Regnase-1 (also known as Zc3h12a and MCPIP1) is an RNase whose expression level is stimulated by lipopolysaccharides and prevents autoimmune diseases by directly controlling the stability of mRNAs of inflammatory genes such as interleukin (IL)-6, IL-1β, IL-2, and IL-12p404567. Regnase-1 accelerates target mRNA degradation via their 3′-terminal untranslated region (3′UTR), and also degrades its own mRNA8. Regnase-1 is a member of Regnase family and is composed of a PilT N-terminus like (PIN) domain followed by a CCCH-type zinc–finger (ZF) domain, which are conserved among Regnase family members. Our findings suggest that Regnase-1 cleaves its target mRNA by an NTD-activated functional PIN dimer, while the ZF increases RNA affinity in the vicinity of the PIN dimer.

X-ray crystallography was attempted for the fragment containing both the PIN and ZF domains, however, electron density was observed only for the PIN domain, consistent with a previous report on Regnase-1 derived from Homo sapiens. This suggests that the PIN and ZF domains exist independently without interacting with each other. We found that the PIN domain formed a head-to-tail oligomer that was commonly observed in all three crystal forms in spite of the different crystallization conditions. The amino acid sequences corresponding to PIN (residues 134–295) are the two non-identical residues are substituted with similar amino acids. Both the mouse and human PIN domains form head-to-tail oligomers in three distinct crystal forms. In contrast, our gel filtration data, mutational analyses, and NMR spectra all indicate that the PIN domain forms a head-to-tail dimer in solution in a manner similar to the crystal structure. The previously reported crystal structure of the Regnase-1 PIN domain derived from Homo sapiens is nearly identical to the one derived from Mus musculus in this study, with a backbone RMSD of 0.2 Å. The importance of residues W182 and R183 can readily be understood in terms of the monomeric PIN structure as they are located near to the RNase catalytic site; however, the importance of residue K184, which points away from the active site is more easily rationalized in terms of the oligomeric structure, in which the “secondary” chain’s residue K184 is positioned near the “primary” chain’s catalytic site. In contrast, R214 is important for oligomerization of the PIN domain and the “secondary” chain’s residue R214 is also positioned near the “primary” chain’s active site within the dimer interface. Within the crystal structure of the PIN dimer, the Regnase-1 specific basic regions in both the “primary” and “secondary” PINs are located around the catalytic site of the primary PIN. In the absence of target mRNA, the PIN domain forms head-to-tail oligomers at high concentration.

>GPHMDLRPVVIDGSNVAMSHGNKEVFSCRGILLAVNWFLERGHTDITVFVPSWRKEQPRPDVPITDQHILRELEKKKILVFTPSRRVGGKRVVCYDDRFIVKLAFESDGVVVSNDTYRDLQGERQEWKRFIEERLLMYSFVNDKFMPPDDPLGRHGPSLDNFLRKKPLPSEHRKQPCPYGKKCTYGIKCRFFHPERPSRPQRSVADELRA[4x]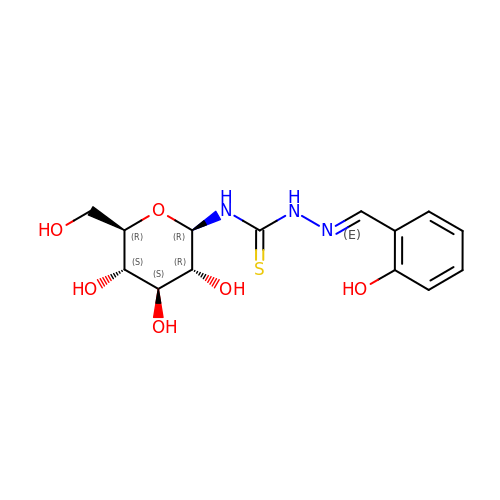N-({(2E)-2-[(2-hydroxyphenyl)methylidene]hydrazino}carbonothioyl)-beta-D-glucopyranosylamine | C14 H19 N3 O6 S | YXAUMHVOUHQJAX-IVSPNHRTSA-N4-(5-AMINO-4-OXO-4H-PYRAZOL-3-YL)-2-BROMO-4,5,6,7-TETRAHYDRO-3AH-PYRROLO[2,3-C]AZEPIN-8-ONE | C11 H10 Br N5 O2 | 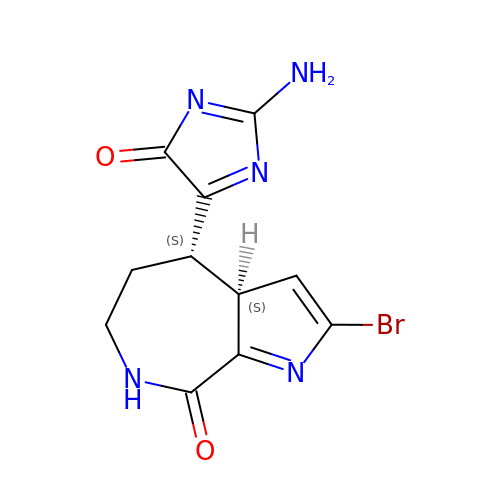QPCBNXNDVYOBIP-WHFBIAKZSA-N> TRDRVPTYQYNMNFEKLGKCIIINNKNFDKVTGMGVRNGTDKDAEALFKCFRSLGFDVIVYNDCSCAKMQDLLKKASEEDHTNAACFACILLSHGEENVIYGKDGVTPIKDLTAHFRGARCKTL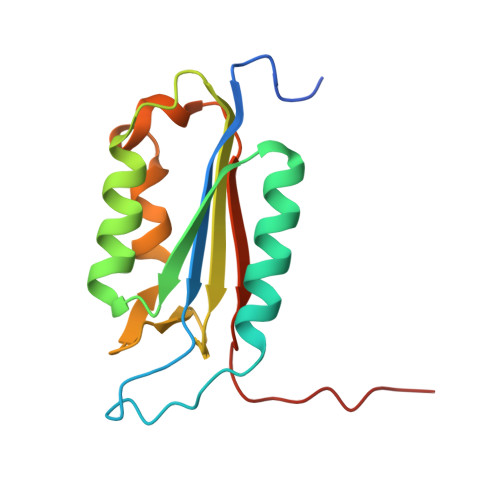LEKPKLFFIQACRGTELDDGIQAD> FACKTANGTAIPIGGGSANVYVNLAPAVNVGQNLVVDLSTQIFCHNDYPETITDYVTLQRGSAYGGVLSSFSGTVKYNGSSYPFPTTSETPRVVYNSRTDKPWPVALYLTPVSSAGGVAIKAGSLIAVLILRQTNNYNSDDFQFVWNIYANNDVVVPTGGCDVSARDVTVTLPDYPGSVPIPLTVYCAKSQNLGY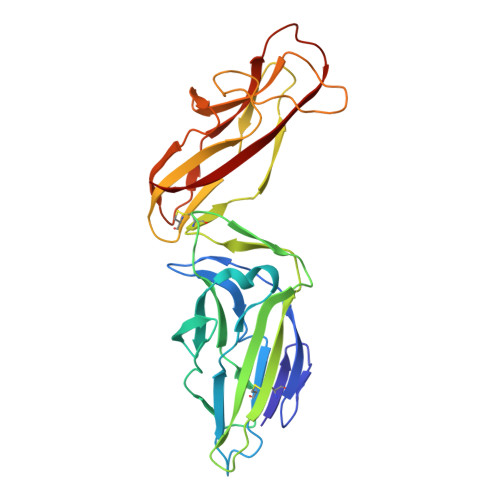YLSGTTADAGNSIFTNTASFSPAQGVGVQLTRNGTIIPANNTVSLGAVGTSAVSLGLTANYARTGGQVTAGNVQSIIGVTFVYQ Dystrophin is a cytoskeletal protein belonging to the spectrin superfamily and is responsible for linking the extracellular matrix (ECM)-binding dystroglycan complex to the cortical actin cytoskeleton. Actin binding by dystrophin is mediated by two portions of the protein: the tandem calponin homology (CH) actin-binding domain 1 (ABD1, residues 1–246) and a series of spectrin repeats (SR) in the middle of the protein comprised of SR11–SR17 and referred to as actin-binding domain 2 (ABD2; residues Phe1461–Gln2209). The ABD1 of dystrophin is a member of the calponin homology domain superfamily. CH domains are found in a range of actin-binding proteins and consist of approximately 100 amino-acid residues with a characteristic α-helical fold that includes a core three-helix bundle and two flanking helices.

The structure of the N-terminal actin-binding domain of human dystrophin was determined at 1.94 Å resolution. Each chain in the asymmetric unit exists in a ‘closed’ conformation, with the first and second calponin homology (CH) domains directly interacting via a 2500.6 Å2 interface. The positioning of the individual CH domains is comparable to the domain-swapped dimer seen in previous human dystrophin and utrophin actin-binding domain 1 structures. The CH1 domain is highly similar to the actin-bound utrophin structure and structural homology suggests that the ‘closed’ single-chain conformation opens during actin binding to mitigate steric clashes between CH2 and actin. There were four protein molecules in the asymmetric unit. Based on the refinement statistics, the closed-conformation AlphaFold2-derived molecular-replacement model was used for further refinement. This choice was supported by the presence of inter-chain 2Fo − Fc electron density for the linker region connecting CH1 and CH2 in all chains of the asymmetric unit. The structural model shows density for peptide backbone residues 13–244, with most residues exhibiting resolved density for side chains. In domain-swapped dystrophin and utrophin dimers, the linker Gln134–Asn137 in dystrophin forms a helix that is extended away from the CH1 and CH2 domains. In the closed conformation, the helix melts and the linker forms a turn.

>STGLWWEEVEDSYEREDVQKKTFTKWVNAQFSKFGKQHIENLFSDLQDGRRLLDLLEGLTGQKLPKEKGSTRVHALNNVNKALRVLQNNNVDLVNIGSTDIVDGNHKLTLGLIWNIILHWQVKNVMKNIMAGLQQTNSEKILLSWVRQSTRNYPQVNVINFTTSWSDGLALNALIHSHRPDLFDWNSVVSQQSATQRLEHAFNIARYQLGIEKLLDPEDVDTTYPDKKSILMYITSLFQVLPQQVSIE[4x]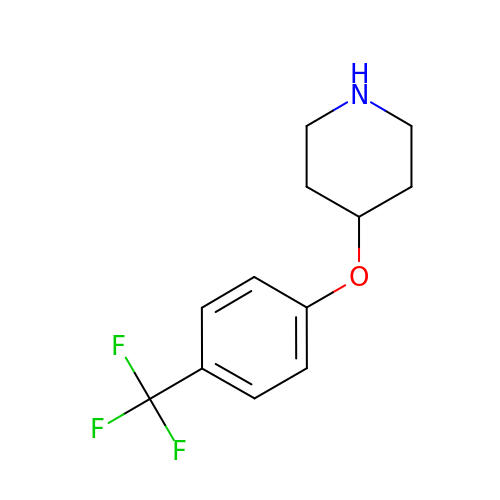4-[4-(trifluoromethyl)phenoxy]piperidine | C12 H14 F3 N O | HRYZQEDCGWRROX-UHFFFAOYSA-N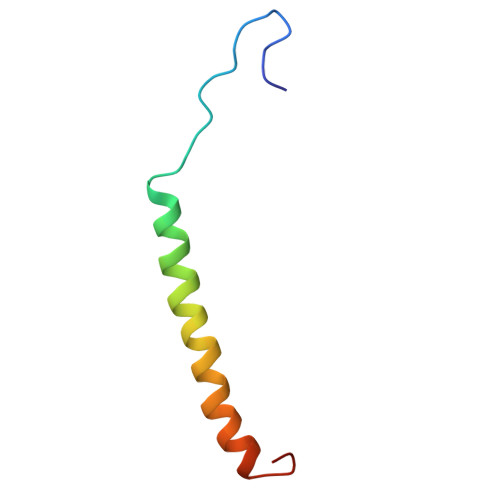> VIVTRSGAILPKPVKMSFGLLRVFSIVIPFLYVGTLISKNFAALLEEHDIFVP Helper NLRs function as central nodes in plant immune networks. Upon activation, they oligomerize into inflammasome-like resistosomes to initiate immune signaling, yet the dynamics of resistosome assembly remain poorly understood. Here, we show that the virulence effector AVRcap1b from the Irish potato famine pathogen *Phytophthora infestans* suppresses immune activation by directly engaging oligomerization intermediates of the tomato helper NLR SlNRC3. Cryo-EM structures of SlNRC3 in AVRcap1b-bound and unbound states reveal that AVRcap1b bridges multiple protomers, stabilizing a stalled intermediate and preventing formation of a functional resistosome.

We captured the effector AVRcap1b from the Irish potato famine pathogen *P. infestans* in complex with stalled three-protomer intermediate of the tomato helper NLR SlNRC3. AVRcap1b interacts with all three SlNRC3 protomers on the interface that, in a fully formed resistosome, would normally be masked by the second half of the hexamer. The effector wraps around the bottom of the three protomers making contact with the underside of the assembled NLRs. The WY1 domain of AVRcap1b, known to contribute to the NbTOL9a binding, was not resolved in our structure suggesting flexibility of this domain that may be important for NbTOL9a engagement. The remaining LWY domains (LWY2-7) collectively form the interface between AVRcap1b and the three SlNRC3 protomers **([Fig fig3])**. Among the LWY domains, LWY6 contributes to the most extensive interaction interface, with a buried surface area of 729 Å^2^, through multiple hydrogen bonds and hydrophobic interactions. Phe207, which plays a crucial role in the LWY6 interaction with protomer-3, also contributes significant buried surface area to the LWY7 interface with protomer-2. Together, LWY6 and LWY7 account for 61% (1274 Å^2^ out of a total of 2088 Å^2^) of the total buried surface area between AVRcap1b and the three SlNRC3 protomers, underscoring their key role in effector binding. Structural analysis of the SlNRC3-AVRcap1b complex revealed that SlNRC3 Tyr204, Glu205, Phe206, and Phe207 (hereafter, the YEFF motif) are simultaneously engaged by LWY6 and LWY7 of AVRcap1b. However, in the presence of AVRcap1b, SlNRC3^Y204A/E205A^ didn’t associate with AVRcap1b in an intermediate band (presumably the 3:1 SlNRC3: AVRcap1b complex) as clearly observed with SlNRC3 (**[Fig fig5]**). These results independently confirm that the Y204A/E205A substitutions disrupt AVRcap1b binding without compromising SlNRC3 resistosome assembly and provides further support for a model in which the effector targets a conserved NB-domain interface to stall resistosome assembly of a helper NLR at a sub-hexameric state (**[Fig fig5]**).

>[3x]MADVAVKFELENETQLEIDNADLILGIQGEVENLLTDLNYFNAFLKEAAKSRRENEVLKELVKKIRKVVNDAEDSIDKFVVEAKRHDDKNKFAQWFHITHVARAKGVADEIKSIRERVKEIRDNDAYGLQAITLDDNFNRGDEERKAPVVEEDDVVGFDDEAKTVIDRLIGGSDYVEVVPVVGMPGLGKTTLAYKIYKDPKVEYEFFTRVWVYVSQTFKRREIFLNIISKFTRNTKQYDDTPEDDLANEVKELLGKGGKYLIVLDDVWTMEAWDRIKIAFPNNGKRNRVLMTTRQSNVAKRCNDKPHDLKFLTKDESWELLEKKVFHKEKCPPELELPGISIAEKCMGLPLAIVVIAGALIGKGKTTREWELVAASVGEHLINRDPENCKKLVQMSYDRLPYDLKACFLYCGAFPGGSQIPAKKLIRLWIAEGFIQYQGPLALEDVAEDHLNDLVNRNLVMVTQRSCSGQIKTCRVHDMLHEFCRHEAMMEENLFQEIKQGQERSFPGKQELATYRRLCIQSLIPEFLSMKPSGEHVRSFLCVGSKKIDMPPNEIPSIPKAFPLLRVLDAESIKFSRFSREFFKLFHLRYIALSTDKIKTIPADFGNLWNIQTLIVETQQATLDIKADIWNMTRLRHVCTNASATLPSTKRPKSSKDNLVNRCLQTLSTIAPECCTAEVFTRTPNLKKLGVRGKIDALLESSKDGSGSGLFSNIGKLGCLEYLKLVNDTRLSSKPLHLPPAYIFPQKLKKLSLVDTWFEWKDMSILGLLPELEVLKLKENAFKGQSWEQEDGGFPRLQVLWIERTDLTSWKASSGNFPRLKHLALISCDKLEELPAELADVKNLQLIELQSSSESAARSARAILKRNQEKEQDGDKGTGFKLSIFPHDLGLSDYKDHDGDYKDHDLDAAAADYKDDDDK;> MAPSIVENIKALVKSSAVTPAKLQQWLDERLEAGLVFKNMNLDEPNIFSLLHEPNFAKWVQYADDLSAKSSHKESSVISTLTSLHGDKVVYDTIQAAKLYPQLSELALKLEKDQIRFWIATRKDPSVVFEALNLNWAGISIFPKPEFSAWLKYVDDVNARHPKEAPLSIIPTLKQRFSRGDEAGTDVLLKLIANGKATTEAKTVANKVESALFDFWLNSRETPDKVMDAFKYGTTTQAFLGSPRWKEWERYLSAYNARYPEKKATAIETLTRKYGDAQLLDTLIGASSKGETKTLAAKLQAQQFDRWMNLKESPLDVYNRLRSSYGDTAFFNEPQLNVWVSYMNVFVDKNPSKVDKMFLELGDTFGDMRLFRVLGEAKKFPNLESTATKLQMEKASTLFASGKSPEGIFKVLALDNVGDDILSNTLFHKWLAYLQKFNKEHPNNQESWFDMLRISYQPFGVERIIETGRKNPLTRLMAEKVENAYHNYWLDIKMEPKTAFRSLHLDESGEKLLADPKFNTWVQYLKTFNDRYPNEKTTVIDGLRDNSHDIALLRMFSAAKNDPSTEKLATDLQSALILKWQDAKKTPEELKRVFVGVPAADEMLDRYIKLLAVASSTPYSYPYDVPDYAGYPYDVPDYAGLYPYDVPDYATRAAYPYDVPDYAGYPYDVPDYAGLYPYDVPDYA>[3x]MHHHHHHHHENLYFQGKTEVAPGVHHVHPLPDSVPESEDLFAPPPRMQGKEGRPKPHIGPNYESYVKEWAKTVGPNSDEWWAAKARETLDWYDDFKTVRAGGFEHGDVQWFPEGTLNAAYNCLDRHYYKNPKKTAIIYEADEPSESREVSYEELMQETCRVANVLKSYGVKKGDAVSIYLPMTWQAAA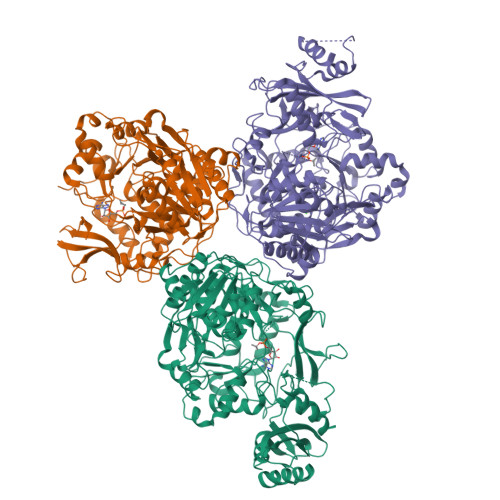AFLACARIGAIHSAVFAGFSAESLRDRVNDCECKVLITTDEGRRGGKTIATKQIVDAALQQCPLVENVLVLRRTGNKVPMTEGRDKWWDEECAKMPAYCPCERMASEDPLFILYTSGSTGKPKGVVHSTAGYLLGTALTLKYVFDAHPDDRFACMADIGWITGHSYIIYGPLANGITTAVFESTPVYPTPSRYWDFVDKWKATQLYTAPTAIRLLRRMGEDHVKNHDLSSLRVLGSVGEPINPEAWHWYNDFAGKNQCAIVDTYWMTETGSISIAPLPGAISTKPGSATFPFFGMDVDIIDPQTGQVLEGNDVEGVLVARRPWPSIARTVYRDHKRYLETYMKPYPGYFFFGDGAARDYDGYMWIKGRVDDVINVSGHRLSTAEVESALILHKGVAETAVVGCADDLTGQAVYAFVTMKPEFDLKATKEADLSKELAIQVRKVIGPFAAPKKIYLVSDLPKTRSGKIMRRVLRKIVAGEGDQLGDLSSIADPQIVEEVKQKVTGSA> SNAVLKIIQGALDTRELLKAYQEEACAKNFGAFCVFVGIVRKEDNIQGLSFDIYEALLKTWFEKWHHKAKDLGVVLKMAHSLGDVLIGQSSFLCVSMGKNRKNALELYENFIEDFKHNAPIWKY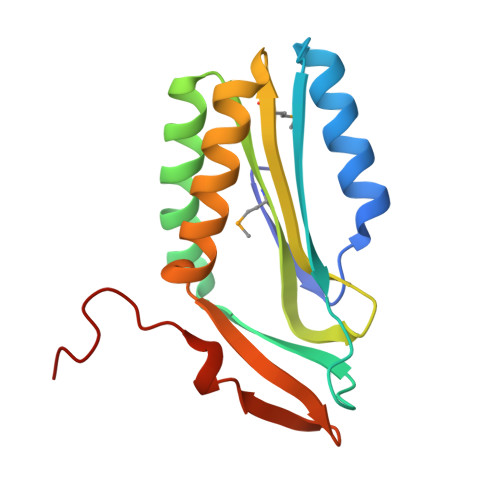DLIHNKRIYAKERSHPLKGSGLLA>[4x]MIFDK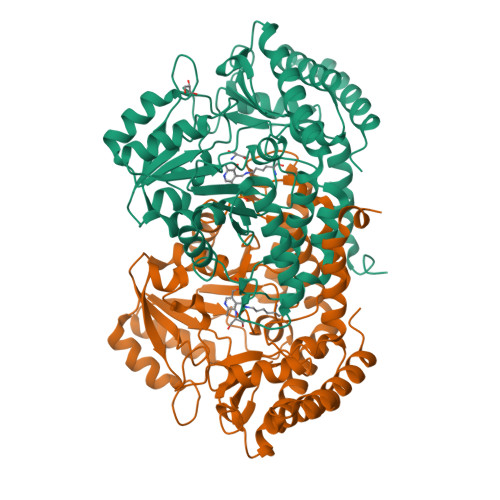EDYKAFDPELWNAIDAEAERQQNNIELIASENVVSKAVMAAQGTLLTNKSAEGYPGKRYYGGTAVIDVVETLAIERAKKLFGAKFANVQPHSGSQANAAVYMSLIQPGDTVMGMDLSAGGHLTHGAPVSFSGKTYNFVSYNVDKESELLDYDAILAQAKEVRPKLIVAGASAYSRIIDFAKFREIADAVGAYLMVDMAHIAGLVASGHHPSPVPYAHVTTTTTHKTLRGPRGGLILTDDEDIAKKLNSAVFPGLQGGPLEHVIAAKAVALKEALDPAFKEYGENVIKNAAAMADVFNQHPDFRVISGGTNNHLFLVDVTKVVENGKVAQNVLEEVNITLNKNSIPYEQLSPFKTSGIRVGSPAITSRGMGEAESRQIAEWMVEALENHDKPEVLERIRGDVKVLTDAFPLY2-(4,6-dimethylpyrimidin-2-yl)-3H-isoindol-1-imine | C14 H14 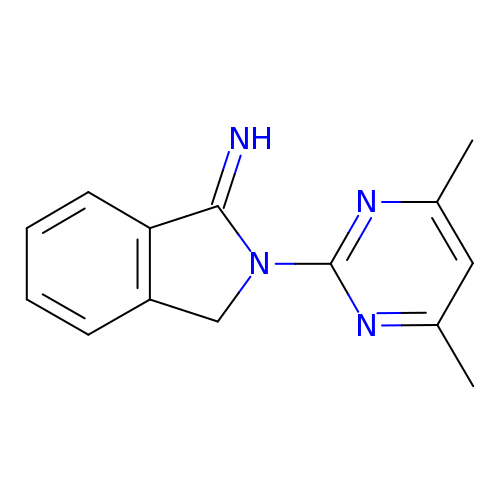N4 | CNIPEVQUYISKFW-UHFFFAOYSA-N> MSSYTGAALAPKSERLRLAFEEKQKDHQKCIEEAKGKGLKKDELIDACAWTHRK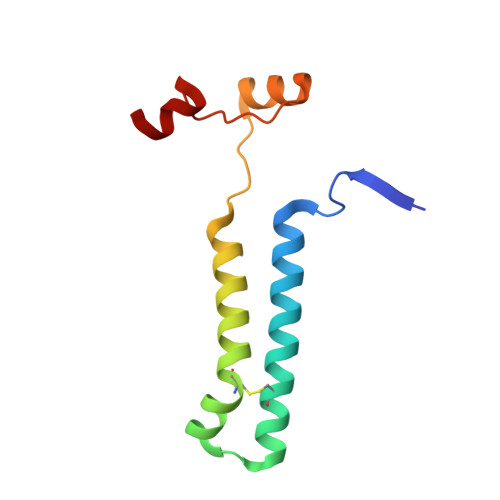TILALKDWFAYRPPFQDRRSKWAEYCSIRHDSGSWLGWSQKFF>[6x]MTDTHTGPTPADAVPAYPFSLPHALDLDPHYAELRRDEPVSRVRLPYGEGTAWLVTRMSDARIVLGDSRFSTAAATDPATPRMFPTPPEPDGVLAQDPPDHTRLRRLVGKAFTARRVEEMRPRVRSLVDSLLDDMVAHGSPADLVEFLAVPFPVAVICELLGVPLEDRDLFRTFSDAMLSSTRLTAAEIQRVQQDFMVYMDGLVAQRRDAPTEDLLGALALATDNDDHLTKGEIVNMGVSLLIAGHET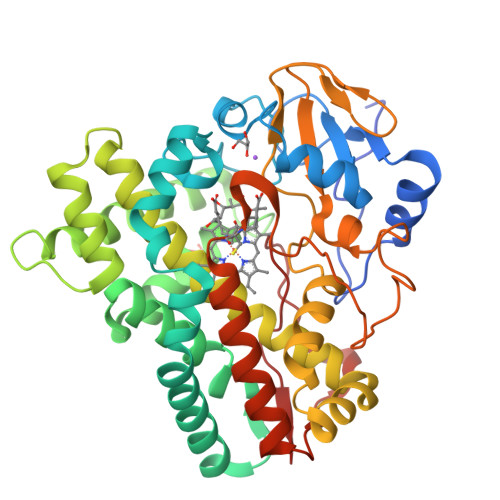SVNQITNLVHLLLTERKRYESLVADPALVPAAVEEMLRYTPLVSAGSFVRVATEDVELSTVTVRAGEPCVVHFASANRDEEVFDHADELDFHRERNPHIAFGHGAHHCIGAQLGRLELQEALSALVRRFPTLDLAEPVAGLKWKQGMLIRGLERQIVSW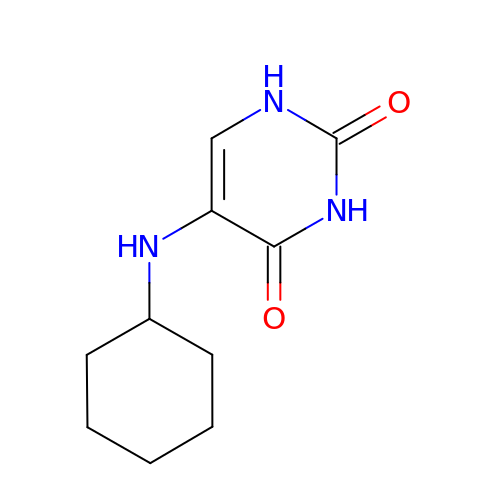5-(cyclohexylamino)pyrimidine-2,4(1H,3H)-dione | C10 H15 N3 O2 | WHMIGQGVTIZZPV-UHFFFAOYSA-N(4~{Z})-2-(1-adamantylamino)-4-(1,3-benzothiazol-6-ylmethylidene)-1~{H}-imidazol-5-one 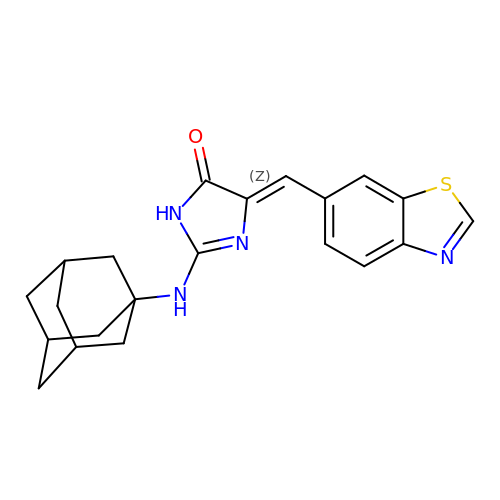| C21 H22 N4 O S | HEVBCYZPXGZFGS-KDBINBPISA-N>MTDTHTGPTPADAVPAYPFSLPHALDLDPHYAELRRDEPVSRVRLPYGEGTAWLVTRMSDARIVLGDSRFSTAAATDPATPRMFPTPPEPDGVLAQDPPDHTRLRRLVGKAFTARRVEEMRPRVRSLVDSLLDDMVAHGSPADLVEFLAVPFPVAVICELLGVPLEDRDLFRTFSDAMLSSTRLTAAEIQRVQQDFMVYMDGLVAQRRDAPTEDLLGALALATDNDDHLTKGEIVNMGVSLLIAGHETSVNQITNLVHLLLTERKRYESLVADPALVPAAVEEMLRYTPLVSAGSFVRVATEDVELSTVTVRAGEPCVVHFASANRDEEVFDHADELDFHRERNPHIAFGHGAHHCIGAQLGRLELQEALSALVRRFPTLDLAEPVAGLKWKQG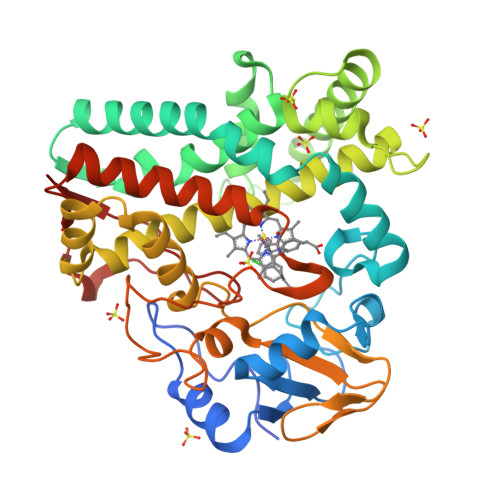MLIRGLERQIVSW[2x]> MRLEFSIYRYNPDVDDAPRMQDYTLEADEGRDMMLLDALIQLKEKDPSLSFRRSCREGVCGSDGLNMNG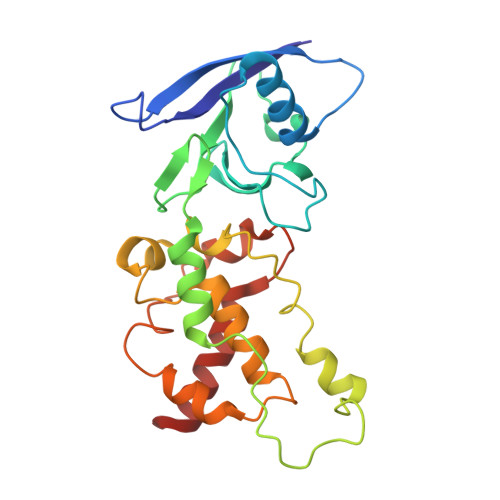KNGLACITPISALNQPGKKIVIRPLPGLPVIRDLVVDMGQFYAQYEKIKPYLLNNGQNPPAREHLQMPEQREKLDGLYECILCACCSTSCPSFWWNPDKFIGPAGLLAAYRFLIDSRDTETDSRLDGLSDAFSVFRCTSIMNCVSVCPKGLNPTRAIGHIKSMLLQRNA> HMLEAKFEEASLFKRIIDGFKDCVQLVNFQCKEDGIIAQAVDDSR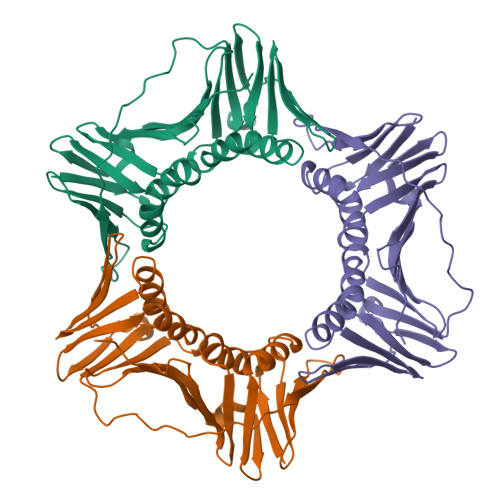VLLVSLEIGVEAFQEYRCDHPVTLGMDLTSLSKILRCGNNTDTLTLIADNTPDSIILLFEDTKKDRIAEYSLKLMDIDADFLKIEELQYDSTLSLPSSEFSKIVRDLSQLSDSINIMITKETIKFVADGDIGGGSVIIKPFVDMEHPETSIKLEMDQPVDLTFGAKYLLDIIKGSSLSDRVGIRLSSEAPALFQFDLKSGFLQFFLAPKFNDEE>WKDKEFQVLFVLTILTLISGTIFYSTVEGLRPIDALYFSVVTLTTVGDGNFSPQTDFGKIF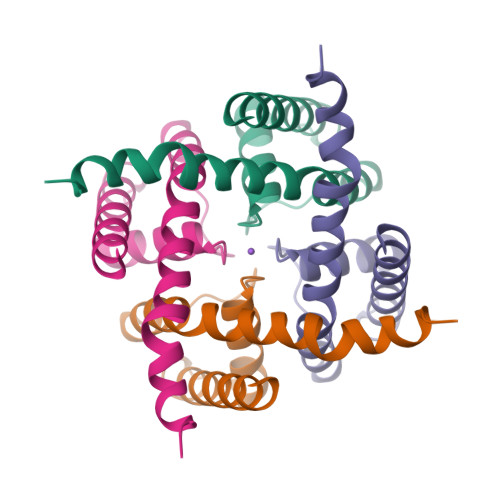TILYIFIGIGLVFGFIHKLAVNVQLPSILSNLVPR[2x]>[2x]GLVPRGSHMKVLVAEDQSMLRDAMCQLLTLQPDVESVLQAKNGQEAIQLLEKESVDIAILDVEMPVKTGLEVLEWIRSEKLETKVVVVTTFKRAGYFERAVKAGVDAYVL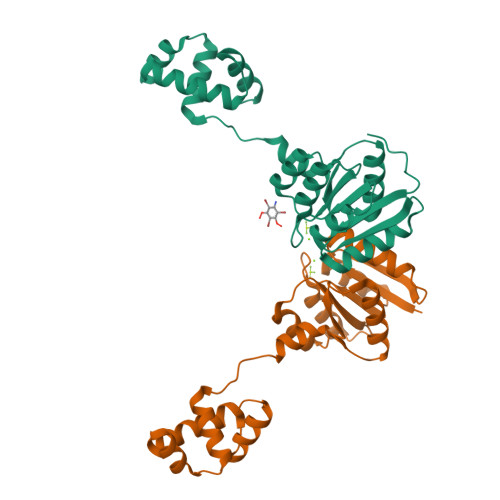KERSIADLMQTLHTVLEGRKEYSPELMEMVMTRPNPLTEQEIAVLKGIARGLSNQEIADQLYLSNGTIRNYVTNILSKLDAGNRTEAANIAKESGWL>[2x]MAEPQPPSGGLTDEAALSCCS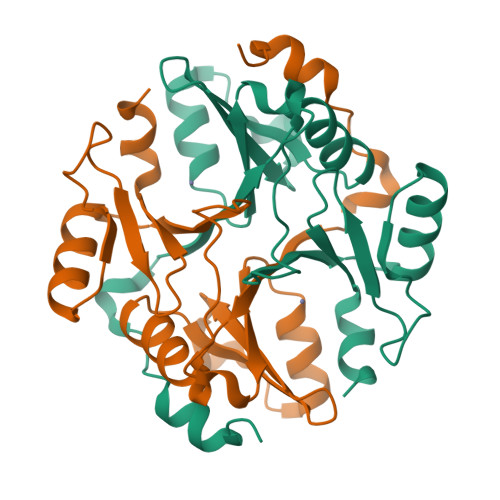DADPSTKDFLLQQTMLRVKDPKKSLDFYTRVLGMTLIQKCDFPIMKFSLYFLAYEDKNDIPKEKDEKIAWALSRKATLELTHNWGTEDDETQSYHNGNSDPRGFGHIGIAVPDVYSACKRFEELGVKFVKKPDDGKMKGLAFIQDPDGYWIEILNPNKMATLMLEHHHHHH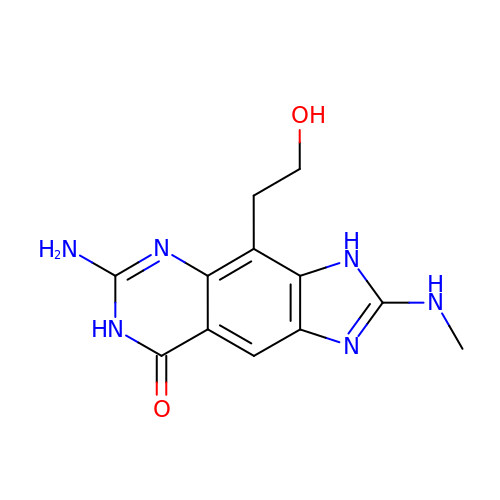6-amino-4-(2-hydroxyethyl)-2-(methylamino)-3,7-dihydro-8H-imidazo[4,5-g]quinazolin-8-one | C12 H14 N6 O2 | VKUWLKQBGXDONE-UHFFFAOYSA-N>MKITNYEIYKLKKSGLTNQQILKVLEYGENVDQELLLGDIADISGCRNPAVFMERYFQIDDAHLSKEFQKFPSFSILDDCYPWDLSEIYDAPVLLFYKGNLDLLKFPKVAVVGSRACSKQGAKSVEKVIQGLENELVIVSGLAKGIDTAAHMAALQNGGKTIAVIGTGLDVFYPKANKRLQDYIGNDHLVLSEYGPGEQPLKFHFPARNRIIAGLCRGVIVAEAKMRSGSLITCERAMEEGRDVFAIPGSILDGLSDGCHHLIQEGAKLVTSGQDVLAEF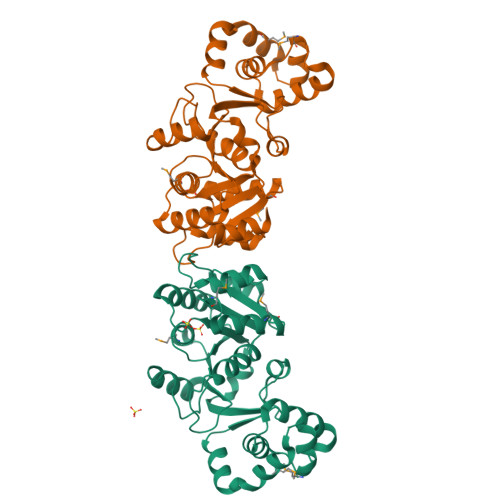EFHHHHHH[3x]> MGSSHHHHHHSSGLVPRGSEMHLLARLAPHLPYIRRYARALTGDQATGDHYVRVALEALAAGELVLDANLSPRVALYRVFHAIWLSSGAQLEVGHDQGLHAGDDAAQRLMRIAPRSRQAFLLTALEGFTPTEAAQILDCDFGEVERLIGDAQAEIDAELATEVLIIEDEPVIAADIEALVRELGHDVTDIAATRGEALEAVTRRTPGLVLADIQLADGSSGIDAVKDILGRMDVPVIFITAFPERLLTGERPEPTFLITKPFQPETVKAAIGQALFFHP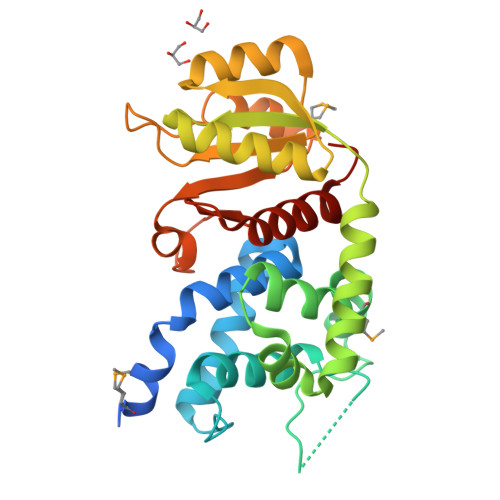RRTAKAA>LTAKHRPSVVWLHNAECTGCTEAAIRTIKPYIDALILDTISLDYQETIMAAAGEAAEAALHQALEGKDGYYLVVEGGLPTIDGGQWGMVAGHPMIETTKKAAAKAKGIICIGTCSAYGGVQKAKPNPSQAKGVSEALGVKTINIPGCPPNPINFVGAVVHVLTKGIPDLDSNGRPKLFYGELVHDNCPRLPHFEASEFAPSFDSEEAKKGFCLYELGCKGPVTYNNCPKVLFNQVNWPVQAGHPCLGCSEPDFWDTMTPFYEQG[6x];>[6x]MAESKPTPQSTFTGPIVVDPITRIEGHLRIMVEVENGKVKDAWSSSQLFRGLEIILKGRDPRDAQHFTQRACGVCTYVHALASSRCVDDAVKVSIPANARMMRNLVMASQYLHDHLVHFYHLHALDWVDVTAALKADPNKAAKLAASIAPARPGNSAKALKAVQDKLKAFVESGQLGIFTNAYFLGGHKAYYLPPEVNLIATAHYLEALHMQVKAASAMAILGGKNPHTQFTVVGGCSNYQGLTKDPLANYLALSKEVCQFVNECYIPDLLAVAGFYKDWGGIGGTSNYLAFGEFATDDSSPSKHLAT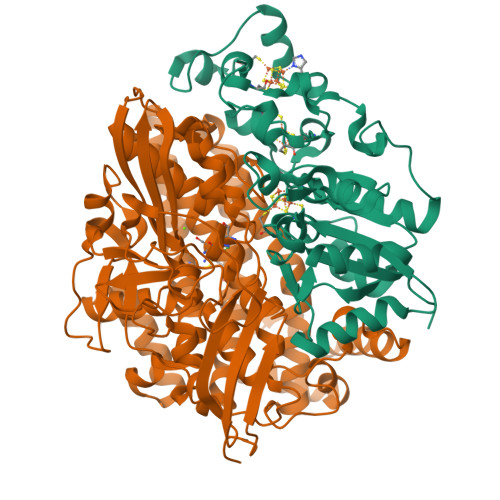SQFPSGVITGRDLGKVDNVDLGAIYEDVKYSWYAPGGDGKHPYDGVTDPKYTKLDDKDHYSWMKAPRYKGKAMEVGPLARTFIAYAKGQPDFKKVVDMVLGKLSVPATALHSTLGRTAARGIETAIVCANMEKWIKEMADSGAKDNTLCAKWEMPEESKGVGLADAPRGALSHWIRIKGKKIDNFQLVVPSTWNLGPRGAQGDKSPVEEALIGTPIADPKRPVEILRTVHAFDPCIACGVH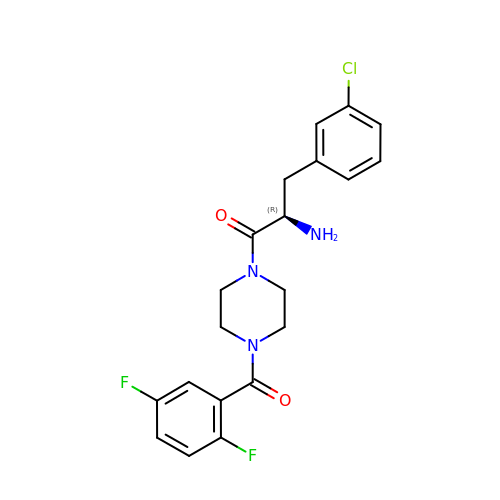(2R)-2-amino-3-(3-chlorophenyl)-1-[4-(2,5-difluorobenzoyl)piperazin-1-yl]propan-1-one | C20 H20 Cl F2 N3 O2 | NASCAWUSOSJBJH-GOSISDBHSA-N>[2x]MTKQEKIEKTITFVKHILEKDASGHDWYHIRRVHKMAISLSEQEGGNRFIIEMAALLHDVADEKLNESEEAGMKKVSDWLEELHVEEEES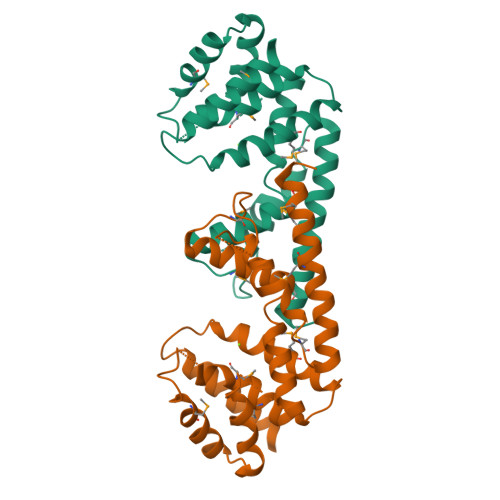KHVLHIIANMSYKGGHGGKVESIEGKLVQDADRLDALGAIGIARTFAYGGAKGRLMYDPTIPPREVMTKDEYRKNNDPSLNHFYEKLLKLKDLMNTNAAKQEAEVRHRYMEQFIEQFMKEWNAQILEHHHHHH2-benzyl-N-cyclopropyl-6-(1-methyl-1H-1,2,3-triazol-4-yl)isonicotinamide 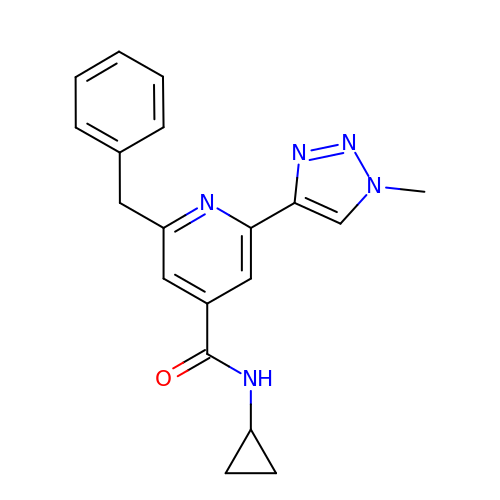| C19 H19 N5 O | NUQGANYMFKALLD-UHFFFAOYSA-N> MASHKLLVTPPKALLKPLSIPNRLLLGPGPSNLPPRIMAAGGLQMIGHMSKEMYQIMDEIKEGIQYVFQTRNPLTLVISGSGHCALEAALVNVLEPGDSFLVGANGIWGQRAADIGERIGARVHPMTKDPGGHYTLQEVEEGLAQHKPVLLFLTHGESSTGVLQPLDGFGELCHRYKCLLLVDSVASLGGTPLYMDRQGIDILYSGSQKALNAPPGTSLISFSDKAKKKMYSRKTKPFSFYLDIKWLANFWGCDDQPRMYHHTIPVISLYSLRESLALIAEQGLENSWRQHREAAAYLHGRLQALGLQLFVKDPALRLPTVTTVAVPAGYDWRDIV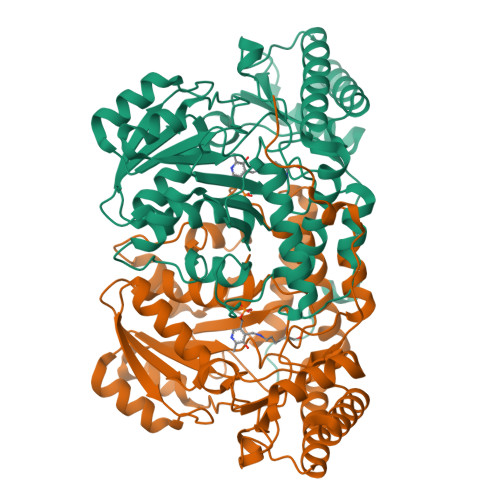SYVMDHFDIEIMGGLGPSTGKVLRIGLLGCNATRENVDRVTEALRAALQHCPKKKL> MELIQDTSRPPLEYVKGVPLIKYFAEALGPLQSFQARPDDLLISTYPKSGTTWVSQILDMIYQGGDLEKCHRAPIFMRVPFLEFKVPGIPSGMETLKNTPAPRLLKTHLPLALLPQTLLDQKVKVVYVARNA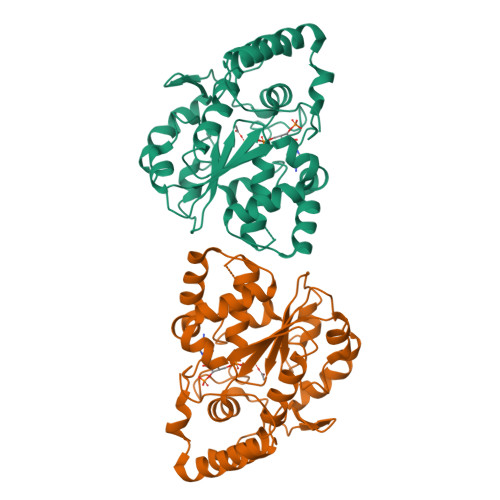KDVAVSYYHFYHMAKVYPHPGTWESFLEKFMAGEVSYGSWYQHVQEWWELSRTHPVLYLFYEDMKENPKREIQKILEFVGRSLPEETVDLMVEHTSFKEMKKNPMTNYTTVRREFMDHSISPFMRKGMAGDWKTTFTVAQNERFDADYAEKMAGCSLSFRSEL> MVNFKDKSMPTAIEKALDFIGGMNTSASVPHSMDESTAKGILKYLHDLGVPVSPEVVVARGEQEGWNPEFT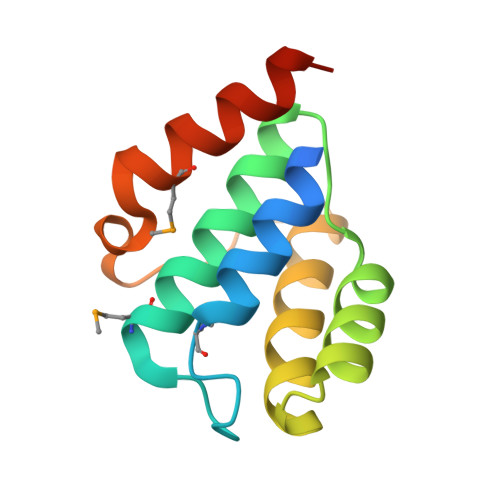KKVAGWAEKVASGNRILIKNPEYFSTYMQEQLKELVLEHHHHHH>STNDNIKDLLDWYSSGSDTFTNSEVLDNSLGSMRIKNTDGSISLIIFPSPYYSPAFTKGEKVDLNTKRTKKSQHTSEGTYIHFQISGVTNTEKLPTPIELPLKVKVHGKDSPLKYWPKFDKKQLAISTLDFEIRHQLTQTHGLYRSSDKTGGYWKITMNDGSTYQSDLSKKFE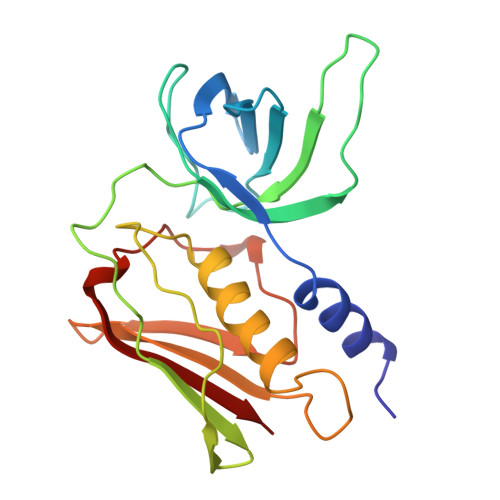YNTEKPPINIDEIKTIEAEIN[2x]> MGHHHHHHHHHHSSGHIEGRHMTTNGADPLGRFSALTREWFTTAFAAPTPAQADAWSAISEGNNTLVIAPTGSGKTLAAFLWAIDRLADPAREPSQGTQVLYVSPLKALAVDVERNLRTPLTGITRVAERHGLPAPSITVGVRSGDTPPNQRRAMIANPPDVLITTPESLFLMLTSAARETLTSVRTVIVDEVHAVAATKRGAHLALSLERLDQLLDTPAQRIGLSATVRPPEEVARFLSGQAPTTIVCPPAAKTFDLSVQVPVPDMANLDNNSIWPDVEERIVDLVEAHNSSIVFANSRRLAERLTSRLNEIHAERSGIELPAGPNPEVGGGAPAHLMGSGQANGAPPLLARAHHGSVSKEQRAQVEDDLKSGRLRAVVATSSLELGIDMGAVDLVIQVEAPPSVASGLQRVGRAGHQVGEISQGVLFPKHRTDLIGCAVTVQRMQTGDIETLRVPANPLDVLAQHTVAVAALEPVDADAWFDAVRRSAPFATLPRSAFEATLDLLSGKYPSTEFAELRPRLVYDRDTGTLTARPGAQRLAVTSGGAIPDRGMFTVYLASETEKPSRVGELDEEMVYESRPGDVISLGATSWRITEITHDRVLVIPAPGQPARLPFWRGDSVGRPAELGAAVGAFTGELASLDRKAFDKRCQKMGFAGYATDNLHQLLREQREATGVVPSDTTFVVERFRDELGDWRVILHSPYGLRVHGPLALAVGRRLRERYGIDEKPTASDDGIIVRLPDSGDTPPGADLFVFDADEIEPIVTAEVGGSALFASRFRECAARALLLPRRHPGKRSPLWHQRQRAAQLLDIARKYPDFPIVLEAVRECLQDVYDVPALIELMHKIAQRRL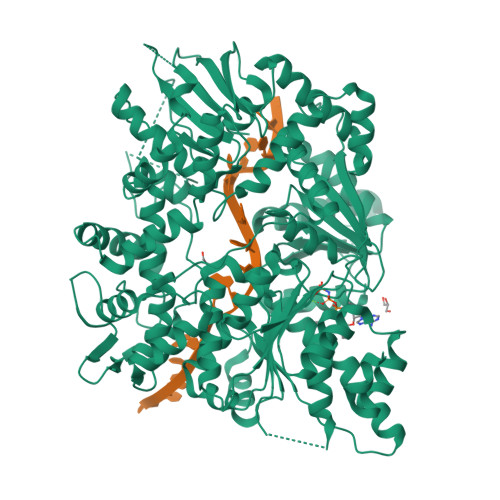RIVEVETATPSPFAASLLFGYVGA Glucokinase (GLK) catalyzes the first reaction in the glycolytic pathway and is a target for regulation in a wide range of organisms. Group II GLKs are ATP-dependent enzymes that lack the classical repressor open reading frame kinase (ROK) sequence motif and contain more than 50 partial and complete protein sequences, including Escherichia coli GLK (ecGLK; Titgemeyer et al., 1994; Meyer et al., 1997). To date, there are no ecGLK structures reported together with the other substrate ATP or the product ADP. This work presents the structure of apo ecGLK bound with phosphate and the structure of ecGLK in complex with both glucose and phosphate, implying a role for phosphate in regulation of the GLK activity. In the ternary complex, phosphate is bound adjacent to glucose, and the B factors for the α4, α5 and α9 helices were further reduced, while r.m.s.d. spikes were observed at the end of the β10 sheet and within the α6 helix of the β-domain. This structural characterization suggests that phosphate could influence the activity of GLK by altering glucose binding and modulating interactions with a loop-interacting regulatory protein.

Here, we report the crystal structure of Escherichia coli glucokinase (GLK), which has phosphate bound in the cleft between the α and β domains adjacent to the active site. The phosphate-bound ecGLK structure from the P43212 crystal form was determined by molecular replacement and refined to an R factor of 0.1930 (Rfree = 0.2302) at a resolution of 2.65 Å. The phosphate-bound complex is composed of a dimer, with each monomer featuring an α/β domain characterized by noncontiguous segments: the small domain (residues 2–110 and 300–321) and the large domain (residues 111–299). The phosphate-binding site is found on the edge of the small and large domain cleft outside the α4–α10 cluster. Arg286 is also important for stabilization through phosphate interaction and undergoes significant structural changes upon binding. The guanidinium group of Arg286 moves closer to the phosphate, allowing the formation of several stabilizing hydrogen bonds. His183, Ser185 and Glu187 exhibit distinct conformational changes upon phosphate binding. Diffraction data were collected at 2.63 Å resolution for the phospate-bound form (Rwork/Rfree = 0.191/0.230) and at 2.54 Å resolution for the ternary complex (Rwork/Rfree = 0.202/0.258), both at 297 K. A B-factor analysis of the phosphate-bound GLK structure revealed consistently lower values for phosphate-interacting basic residues in the α4, α5 and α9 helices, while significant root-mean-square deviation (r.m.s.d.) spikes indicated flexibility in regions preceding β1 and within the loop between the β5 and β6 sheets of the α domain.

>[2x]MTKYALVGDVGGTNARLALCDIASGEISQAKTYSGLDYPSLEAVIRVYLEEHKVEVKDGCIAIACPITGDWVAMTNHTWAFSIAEMKKNLGFSHLEIINDFTAVSMAIPMLKKEHLIQFGGAEPVEGKPIAVYGAGTGLGVAHLVHVDKRWVSLPGEGGHVDFAPNSEEEAIILEILRAEIGHVSAERVLSGPGLVNLYRAIVKADNRLPENLKPKDITERALADSCTDCRRALSLFCVIMGRFGGNLALNLGTFGGVFIAGGIVPRFLEFFKASGFRAAFEDKGRFKEYVHDIPVYLIVHDNPGLLGSGAHLRQTLGHILHHHHHH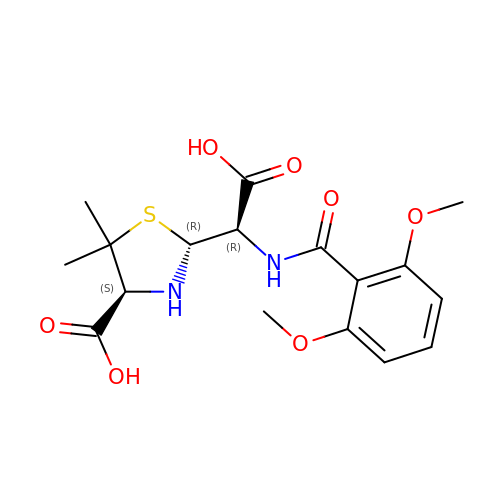(2R,4S)-2-{(R)-carboxy[(2,6-dimethoxybenzoyl)amino]methyl}-5,5-dimethyl-1,3-thiazolidine-4-carboxylic acid | C17 H22 N2 O7 S | JTBCYLJHKDNILB-SGMGOOAPSA-N The FtsEX complex is a widely conserved regulator of peptidoglycan (PG) hydrolases. Instead, it functions as a transmembrane signal transduction system for activating PG hydrolases. Briefly, the ATPase activity by the cytoplasmic FtsE powers the system through its ATP cycle, interacting with the transmembrane FtsX. The signal is then transmitted from the cytosolic FtsE to the two extracellular loops of FtsX via conformational changes, and finally to the coiled-coil (CC) domain proteins.

Next, we used cryo-EM to determine the structure of the FtsEX-RipC complex. The final map achieved a resolution of 3.9 Å. This allowed us to construct a complete model of the complex between FtsE, FtsX, and RipC. The lip of RipC, as well as its adjacent α1 region (residues 102-109) and α2 region (residues 129-148), bind directly to the ECD of FtsX, resulting in a buried surface area of ~1850 Å2. This binding involves three major interfaces that are dominated by extensive hydrophobic interactions, two of which involve a Phe cluster consisting of four phenylalanine residues (F61, F110, F113, and F122) from each of the two lower lobes of the ECD domains. In contrast, RipC is inserted into the ECD domain from the side at a ~116° tilt from the central axis, resulting in an inclined binding mode. When RipC binds, there is an asymmetric response from ECD domains; one ECD domain remains stationary while the other rotates significantly to tightly lock RipC underneath. After RipC recruitment, the two hook-like ECD domains become perpendicular to each other, along with the small loop and top region of TM helices, forming a joint cavity that locks RipC inside. In short, the mechanism of RipC binding involves a “match and fit” process, where one ECD matches and interacts with residues from α1, while the other ECD fits and rotates to lock α2 of RipC underneath. In the ATP-free state, the bound RipC was tilted at ~116°, with the NlpC/P60 domain being well-folded and grasped by the tweezers-like CCD domain and pro-rich linker that is specifically restrained by the N-terminal residues of α1.

>MMITLDHVTKQYKSSARPALDDINVKIDKGEFVFLIGPSGSGKSTFMRLLLAAETPTSGDVRVSKFHVNKLRGRHVPKLRQVIGCVFQDFRLLQQKTVYDNVAFALEVIGKRTDAINRVVPEVLETVGLSGKANRLPDELSGGEQQRVAIARAFVNRPLVLLADEPTGNLDPETSRDIMDLLERINRTGTTVLMATHDHHIVDSMRQRVVELSLGRLVRDEQRGVYGMDR[2x];>MRFGFLLNEVLTGFRRNVTMTIAMILTTAISVGLFGGGMLVVRLADSSRAIYLDRVESQVFLTEDVSANDSSCDTTACKALREKIETRSDVKAVRFLNRQQAYDDAIRKFPQFKDVAGKDSFPASFIVKLENPEQHKDFDTAMKGQPGVLDVLNQKELIDRLFAVLDGLSNAAFAVALVQAIGAILLIANMVQVAAYTRRTEIGIMRLVGASRWYTQLPFLVEAMLAATMGVGIAVAGLMVVRALFLENALNQFYQANLIAKVDYADILFITPWLLLLGVAMSGLTAYLTLRLYVRR[2x];> MRLDQRWLIARVIMRSAIGFFASFTVSSGVLAANVLADPADDALAKLNELSRQAEQTTEALHSAQLDLNEKLAAQRAADQKLADNRTALDAARARLATFQTAVNKVAAATYMGGRTHGMDAILTAESPQLLIDRLSVQRVMAHQMSTQMARFKAAGEQAVKAEQAAAKSAADARSAAEQAAAVRANLQHKQSQLQVQIAVVKSQYVALTPEERTALADPGPVPAVAAIAPGAPPAALPPGAPPGDGPAPGVAPPPGGMPGLPFVQPDGAGGDRTAVVQAALTQVGAPYAWGGAAPGGFDCSGLVMWAFQQAGIALPHSSQALAHGGQPVALSDLQPGDVLTFYSDASHAGIYIGDGLMVHSSTYGVPVRVVPMDSSGPIYDARRY> GHMNMSQSQEIVLQPRSIVVPGELLAEGEFQIPWSPYILKINSKYYSTVVGLFDVKDTQFEVIPLEGSFYYPKINDIVIGLVEDVEIYGWVVDIKAPYKAYLPASNLLGRSINVGEDLRRYLDVGDYVIARIENFDRS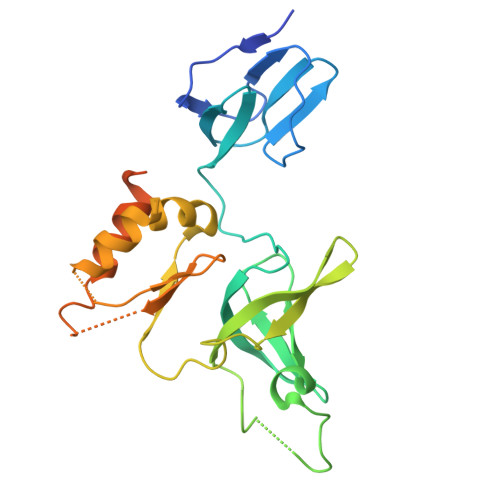IDPVLSVKGKDLGRVSNGIVIDIMPVKVPRVIGKNKSMYETLTSKSGCSIFVANNGRIWATCPSRFSEEILIEAIRKIENESHIKGLTDRIKQFIEEKLGERNASSGETKTNS>[2x]GSSHHHHHHSGDPASMNNHPEVKIK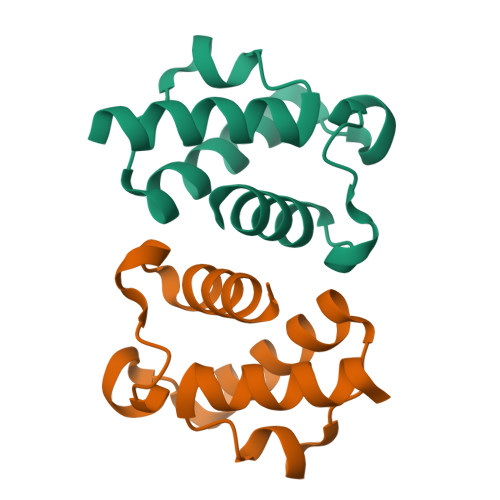TILSLFLNINIDDFNMDANLADAYDMDSTELADLAKEIEKEFGISVTKSQFSHWETGRAVLDFVSSSLNDKN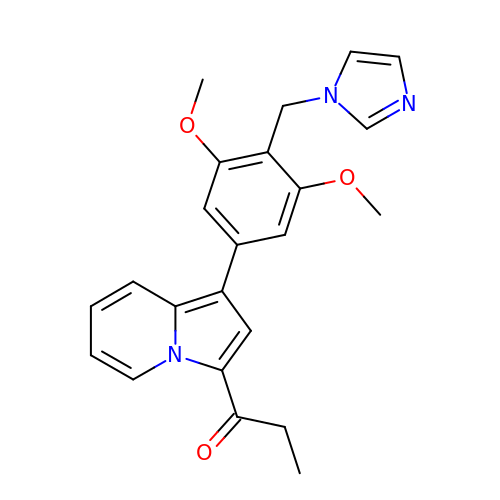1-[1-[4-(imidazol-1-ylmethyl)-3,5-dimethoxy-phenyl]indolizin-3-yl]propan-1-one | C23 H23 N3 O3 | HNTMUAFBKMLFSP-UHFFFAOYSA-N> GSPHMTKAEKILARFNELPNYDLKAVCTGCFHDGFNEVDIEILNQLGIKIFDNIKETDKLNCIFAPKILRTEKFLKSLSFEPLKFALKPEFIIDLLKQIHSKKDKLSQININLFDYEINGINESIISKTKLPTKVFERANIRCINL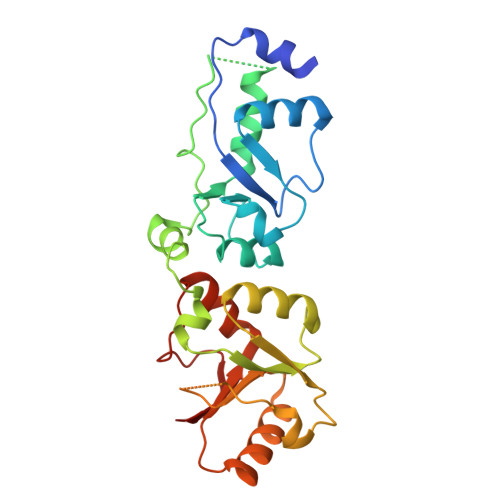VNDIPGGVDTIGSVLKAHGIEKINVLRSKKCTFEDIIPNDVSKQENGGIFKYVLIVTKASQVKKFTKLINDRDKNETILIVEWNWCVESIFHLNVDFTSKKNVLYQKKNN>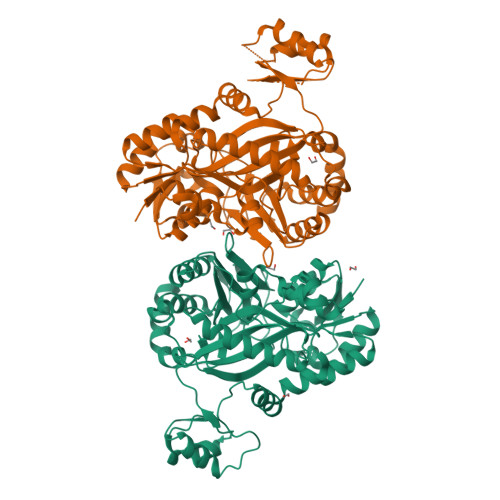[2x]MAHHHHHHHHHHKLTSLYKKAGLENLYFQGMTPRVLIANRGEVAVRIERAVSALGWQSVAVYAPDDAGSLHVRRADEAVALSGRGAAAYLDGAALLRVAQEHAATHVHPGYGFLSENADFARACAQAGLVFVGPDPDTLDLFGDKSRARGLAQRLGVPVIPGTDGATTLEEAAAFMQAQGGAPVMLKACSGGGGRGMRVVRQAGDLAAAFEQASREARLAVGQGDLYAERLIERARHIEVQVAGDGQSVTHLWERDCTVQRRHQKLLEFAPAPHLPQAVRTALIGAALQLAQEVKYRCLGTFEFLVTPGGDFYFIEANPRLQVEHTVTEEWCGTDLVTAQLRLAAGETLTAVGLATQPADAAPPPGQAVQARVNMETLGADGQVHVGGGQVQTFTPPGGPGVRVDTFVTTGLTPSPQYDALLAKVVVHRRDAALPGLLRQAATALSEFQIAGVSTNLAFLQALLHHPDVQHYELSTHWLDERLPELVTQAAEYD1-[bis(4-fluorophenyl)methyl]-4-(1H-1,2,4-triazol-1-ylcarbonyl)piperazine | C20 H19 F2 N5 O | 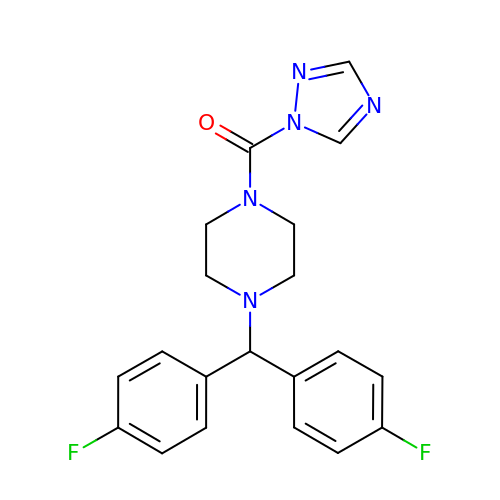UIOVHJYJUUSVIG-UHFFFAOYSA-N>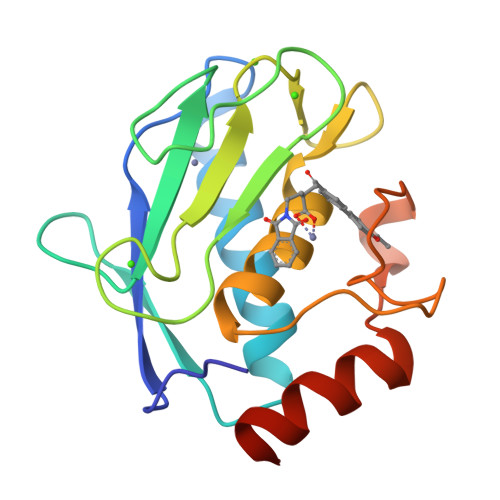[2x]GPVWRKHYITYRINNYTPDMNREDVDYAIRKAFQVWSNVTPLKFSKINTGMADILVVFARGAHGDFHAFDGKGGILAHAFGPGSGIGGDAHFDEDEFWTTHSGGTNLFLTAVHEIGHSLGLGHSSDPKAVMFPTYKYVDINTFRLSADDIRGIQSLYGDPKEN Nogalamycin RO | C35 H41 N O14 | 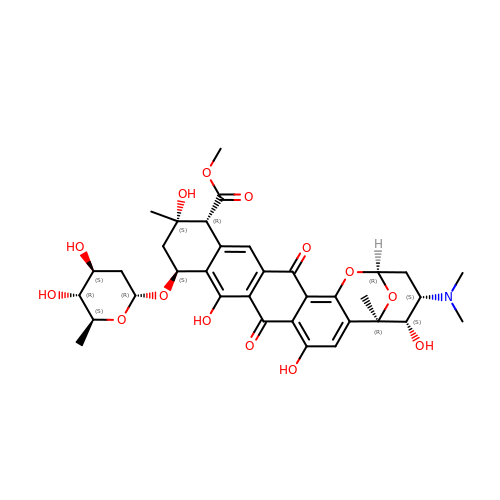CRWWSIJFHVGVFW-PDUKGOLSSA-N> AQNNPYLFRSNKFLTLFKNQHGSLRLLQRFNEDTEKLE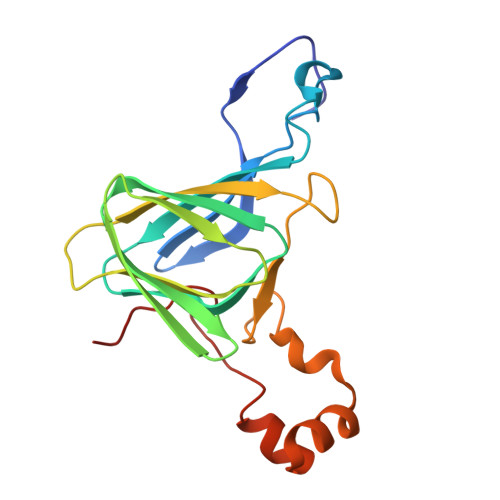NLRDYRVLEYCSKPNTLLLPHHSDSDLLVLVLEGQAILVLVNPDGRDTYKLDQGDAIKIQAGTPFYLINPDNNQNLRILKFAITFRRPGTVEDFFLSSTKRLPSYLSAFSKNFLEASYDSPYDEIEQTLLQEEQEGVIVKMPK>[12x]GKVYKKVELVGTSEEGLEAAIQAALARARKTLR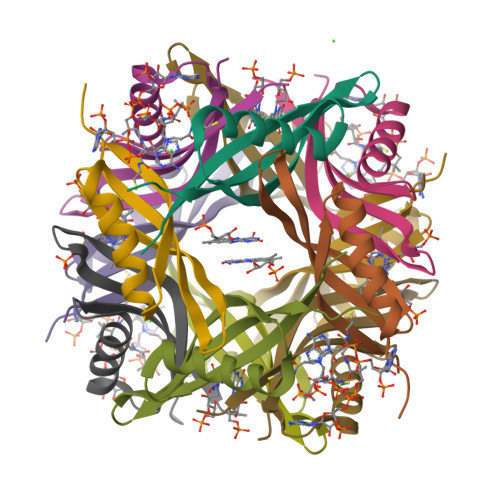HLDWFEVKEIAGTIGEAGVKEYQVVLEVGFRLEET>[18x]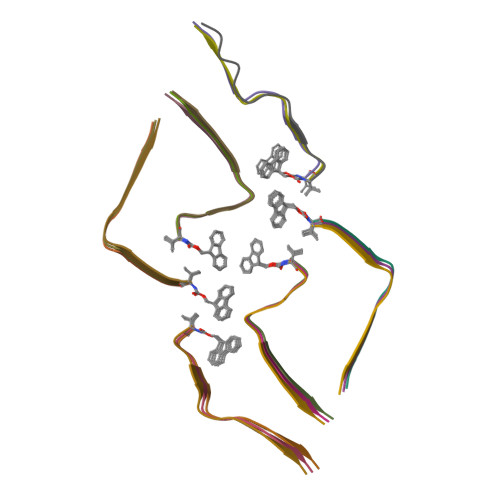XVQSKIGSLDNITHX Glucuronoyl esterases (GEs) within the carbohydrate esterase family 15 (CE15) esterase family, in a range of aerobic and anaerobic fungi and bacteria, have been identified as playing an important role in breaking down LCCs by cleaving the ester bond between 4-O-methyl-d-glucuronyl in xylan and alcohol groups in lignin. GEs share an invariant Ser-His-Glu/Asp catalytic triad and employ a conserved catalytic mechanism that involves the formation of an acyl-enzyme covalent intermediate, which is subsequently cleaved through acid-base hydrolysis. Rumen GEs adopt a canonical α/β hydrolase fold: FsCE15, PrCE15, and RfCE15 adopted the canonical α/β-hydrolase fold that is seen in all of the GE structures solved to date. The fold of all three enzymes consists of a central twisted 10 stranded mixed β-sheet flanked by α-helices on either side.

Crystals of PrCE15 belonged to space group P61 with a single protein molecule in the asymmetric unit. The structure of PrCE15 was refined to Rwork/Rfree of 22.9%/26.9% using data with a maximum resolution of 2.54 Å. A similar examination of these resides in PrCE15 putatively identifies the catalytic residues as Ser226, His355, and Glu249. The catalytic residues of FsCE15 and PrCE15 are positioned in the canonical conformation characteristic of CE15-B subfamily with the general acid located on a loop at the end of β7. FsCE15 and PrCE15 have a conserved disulfide bond between residues Cys345 - Cys483 and Cys225 - Cys356, respectively, which anchors the general base within optimal hydrogen bonding distance (2.7 Å) to the catalytic serine. The arginine following the catalytic serine in the motif contributes to the stabilization of the transition state, and while the arginine is conserved in FsCE15 it is replaced with a tyrosine in PrCE15. Interestingly, it was more common for this residue to be tyrosine in AGF GEs (26 out of 35 sequences) with arginine found at this position in the nine remaining rumen enzymes. PrCE15 displayed a multiphasic unfolding curve however, upon reduction of the disulfide bond, PrCE15 unfolding was monophasic with the higher Tm unfolding event no longer detectable. We determined apparent steady state kinetic parameters for PrCE15 and RfCE15. Both enzymes displayed similar affinities for BnzGlcA; with PrCE15 and RfCE15 having apparent Km values of 5.0 ± 0.4 mM and 6.0 ± 0.4 mM, respectively. The apparent kcat of PrCE15 was determined to be 22.3 ± 0.7 s-1, compared to an apparent kcat of 91.2 ± 0.8 s-1 for RfCE15.

>[2x]MHHHHHHITSLYKKAGMAEVPLVYPKENMGESCKAPTLPQPASCPSVPKLPDPFEWSDGSGRVKNLADWECRRNEIKAEIENYELGKKPAPPQSLKATYSGGTLTVVVNDNGGSLTLTSKISVPSGSGPFPVIIGMNSNTGSLSAGQFSDFIQVPFNHDQCAQYSMTGQKNTNAPFYKLYPNLRDAGDYIAWSWGISRLIDGIEQVKDQIHADMNHIGVTGCSYAGKMALFGGAFDERVALTIPQESGGGGINAWRVSDTIGNVEKIDNTNYSWFMQALKNNFNGKSDKLPYDHHELIAMVAPRAFFTMGNPDYEWLGDKSGYTSAMAALEVWKAMGVEDRFGFNFVGGHMHCSAAGTQVNDVNKFIDRFLRGKSVSTSNMLSSSVTNDYNSWIAAWKGYTIDTSSTTTTPEDPAFLYKV>[2x]GMSVPTLPTGPTVDLAQAAERLIKGRRAVRAFRPDEVPEETMRAVFELAGHAPSNSNTQPWHVEVVSGAARDRLAE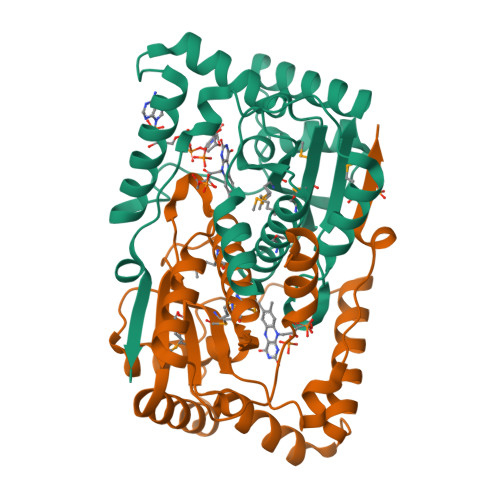ALVTAHAEERVTVDFPYREGLFQGVLQERRADFGSRLYAALGIARDQTDLLQGYNTESLRFYGAPHVAMLFAPNNTEARIAGDMGIYAQTLMLAMTAHGIASCPQALLSFYADTVRAELGVENRKLLMGISFGYADDTAAVNGVRIPRAGLSETTRFSR> GPNEQVSRSQQRGLRRVRDLCRVLQLPPTFEDTAVAYYQQAYRHSGIRAARLQKKEVLVGCCVLITCRQHNWPLTMGAICTLLYADLDVFSSTYMQIVKLLGLDVPSLCLAELVKTYCSSFKLFQASPSVPAKYVEDKEKMLSRTMQLVELANETWLVTGRHPLPVITAATFLAWQSLQPADRLSCSLARFCKLANVDLPYPASSRLQELLAVLLRMAEQLAWLRVLRLDKRSVVKHIGDLLQHRQSLVRSAFRDGTAEVETREKEPPGWGQGQGEGEVGNNSLGLPQGKRPASPALLLPPCMLKSPKRICPVPPVSTVTGDENISDSEIEQYLRTPQEVRDFQRAQAARQAATSVPNPP;> GPSGIVPQLQNIVSTVNLGCKLDLKTIALRARNAEYNPKRFAAVIMRIREPRTTALIFSSGKMVCTGAKSEEQSRLAARKYARVVQKLGFPAKFLDFKIQNMVGSCDVKFPIRLEGLVLTHQQFSSYEPELFPGLIYRMIKPRIVLLIFVSGKVVLTGAKVRAEIYEAFENIYP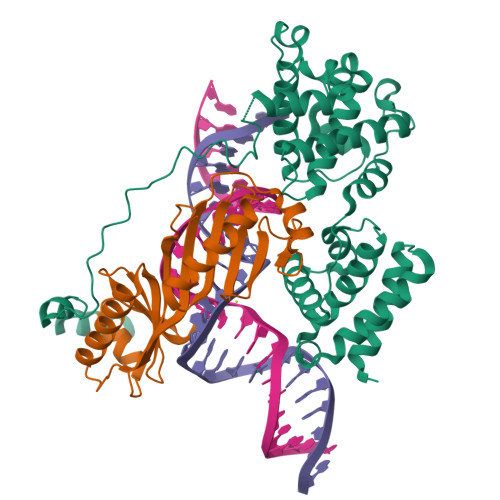ILKGFRKTT>[8x]MHFETTKDGFTIAIGNRIILSHSPDKPAFFAGFGEERMDMYRGNFDIEDYVIERTALRHAEVSGDSVTLSSAPGQAPRLRLTLDGNAIRLTALDETINRLWLRVVAETDEHVWGGGEQMSYFDMRGRRFPLWTSEPGVGRDKTTEITFKSDVSGKAGGDYYNTNYPQPTWLSSRKYALHVETSAYSVFDFRNGDFHEIEIWAVPEKIEFFAGDSFADIVSALSLHFGRQPELPDWVYNGAIIGLKDGVNSFARLEKIRAAGTKVSGLWCEDWVGLRQTSFGARLFWDWQANDTRYPHLRQKIAELADQGIRFLGYVNPYLCVDGPLFPVAESAGYFATDVDGKTAL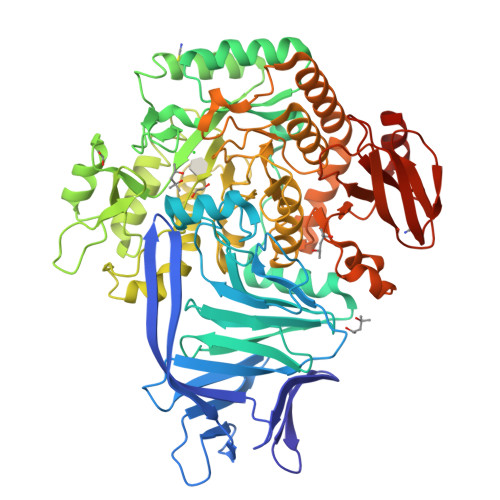VDFGEFDCGVVDFTNPAAADWFAAAIIGKNMLDFGLSGWMADFGEYLPIDIKLSNGVDAKLMHNAWPTLWAEVNAKGVESRGKTGEALFFMRAGFTGVQAHCPLIWGGNQSVDFSRHDGLVTVICGALSSGLMGNAYHHSDIGGYTSLFGNVRTAELIMRWTEMAAFTPVMRTHEGNRPRDNLQIDQDETVLAHFARMTAIYVALAPYLKSLSAEAAKTGLPVQRPLFLHYENEPQTYAVQDCYLYGADMLVAPVWKAGETQRSLYLPGHGEWVHLWSGKRHAGGRDITVETPLGEPAVFYRADSSHHRLFEQLRTIGLEHHHHHH> KDAIEEKFRERLKELVVPKHVMDVVDEELSKLGLLDNHSSEFNVTRNYLDWLTSIPWGKYSNENLDLARAQAVLEEDHYGMEDVKKRILEFIAVSQLRGSTQGKILCFYGPPGVGKTSIARSIARALNREYFRFSVGGMTDVAEIKGHRRTYVGAMPGKIIQCLKKTKTENPLILIDEVDKIGRGYQGDPSSALLELLDPEQNANFLDHYLDVPVDLSKVLFICTANVTDTIPEPLRDRMEMINVSGYVAQEKLAIAERYLVPQARALCGLDESKAKLSSDVLTLLIKQYCRESGVRNLQKQVEKVLRKSAYKIVSGEAESVEVTPENLQDFVGKPVFTVERMYDVTPPGVVMGLAWTAMGGSTLFVETSLRRPQDKDAKGDKDGSLEVTGQLGEVMKESARIAYTFARAFLMQHAPANDYLVTSHIHLHVPEGATPKDGPSAGCTIVTALLSLAMGRPVRQNLAMTGEVSLTGKILPVGGIKEKTIAAKRAGVTCIVLPAENKKDFYDLAAFITEGLEVHFVEH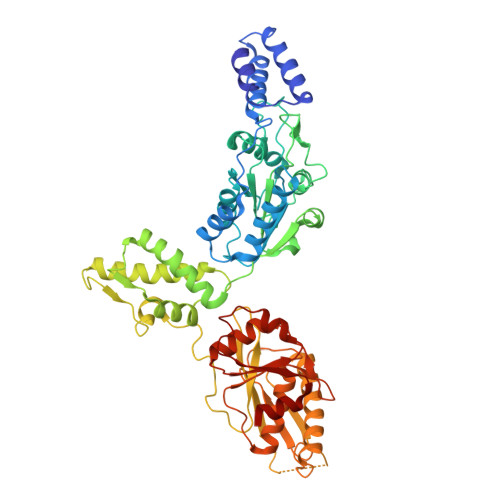YREIFDIAF Enolase (EC 4.2.1.11) is a conserved metalloenzyme present in almost all organisms of the phylogenetic tree that plays a role as a phosphopyruvate hydratase in the reversible chemical reaction of 2-phosphoglycerate (2-PG) to phosphoenolpyruvate (PEP) in the glycolysis pathway (Wold and Ballou, 1957a,b; Reed et al., 1996). Surface enolase is recognized as a plasminogen receptor in several pathogens and is thought to be involved in extracellular matrix degradation and host cell invasion. The assembly of monomer enolase varies among species and is present either as a dimer or octamer but seldom both. Among them, Mycoplasma hyopneumoniae (M. hyopneumoniae, Mhp) is the causative agent of enzootic pneumonia (EP), which is a chronic respiratory disease in pigs and causes significant economic loss in pig production globally.

However, the structure of the enolase of Mycoplasma, which is found in an independent evolutionary branch of bacteria, remains unknown. Here, we reported the first three-dimensional (3D) structure of Mycoplasma enolase (Mhp Eno, short for Mycoplasma hyopneumoniae Enolase). The structure showed a unique Mycoplasma enolase with characteristic long loops in the S3/H1, H6/S6, H7/H8, and H13 regions. As a virulence factor candidate found in our previous studies, Mhp Eno showed a surface localization on M. hyopneumoniae cells as determined by flow cytometry and electron microscopy. Mhp Eno specifically adhered to STECs and recognized the host plasminogen. All of these results show the unique features of Mhp Eno.

>[2x]MSKITKVFAREILDSRGNPTIQVDVYTLAGGFGSAIVPSGASTGSREALELRDTNTKYADNWYGQKGVMTAVDNVNNIIAPEIIGLCCKNQRLIDQKIIELDGTPNKEKLGANAILGVSLAVAKAAANELRMPLFRYLGGTNPTLMPVPMLNVINGGEHASNTLDFQEFMIMPLGFRTFKEALQAANKVFHNLAKLLKKSGFETQVGDEGGFAPNFNSHEQALDFLVDAIKESGFNPGFKGENAVAIAIDAAASEFYNGQKYVFKKLKAASLSKNQADLDEKFEFNSEELLNYYGQLLAKYPIISIEDGFAESDWQGFIAFNQKYGNNHQIVGDDLTVTNVEILKKAINLKAINSILIKLNQIGTLSETLDAIHLAQKSGMTAVISHRSGESEDTTIADLAVAVSSGQIKTGSLSRTDRIAKYNRLLVIEEYLNSYAKADYIGREVFYNLKKLEHHHHHH> SMAAFKPNSINYILGLDIGIASVGWAMVEIDEEENPIRLIDLGVRVFERAEVPKT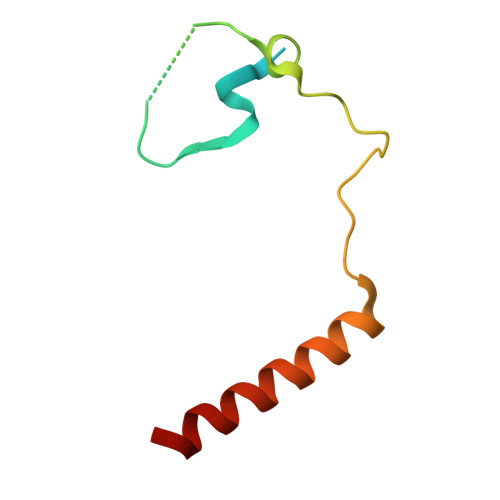GDSLAMARRLARSVRRLTRRRAH>[6x]MFKDGSLIPYLTAGDPD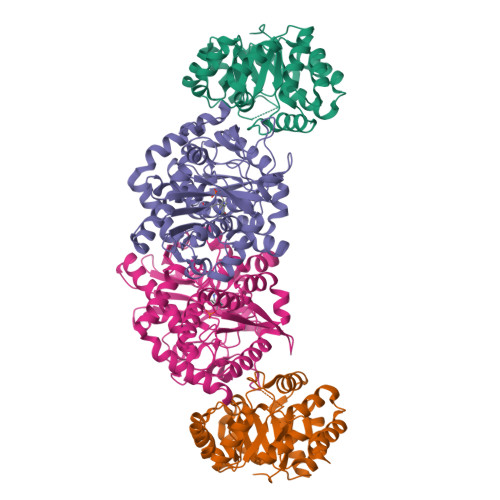KQSTLNFLLALDEYAGAIELGIPFSDPIADGKTIQESHYRALKNGFKLREAFWIVKEFRRHSSTPIVLMTYYNPIYRAGVRNFLAEAKASGVDGILVVDLPVFHAKEFTEIAREEGIKTVFLAAPNTPDERLKVIDDMTTGFVYLVSLYGTTGAREEIPKTAYDLLRRAKRICRNKVAVGFGVSKREHVVSLLKEGANGVVVGSALVKIIGEKGREATEFLKKKVEELLGI;>MWFGEFGGQYVPETLIEPLKELEKAYKRFKDDEEFNRQLNYYLKTWAGRPTPLYYAKRLTEKIGGAKIYLKREDLVHGGAHKTNNAIGQALLAKFMGKTRLIAETGAGQHGVATAMAGALLGMKVDIYMGAEDVERQKMNVFRMKLLGANVIPVNSGSRTLKDAINEALRDWVATFEYTHYLIGSVVGPHPYPTIVRDFQSVIGREAKAQILEAEGQLPDVIVACVGGGSNAMGIFYPFVNDKKVKLVGVEAGGKGLESGKHSASLNAGQVGVFHGMLSYFLQDEEGQIKPTHSIAPGLDYPGVGPEHAYLKKIQRAEYVTVTDEEALKAFHELSRTEGIIPALESAHAVAYAMKLAKEMSRDEIIIVNLSGRGDKDLDIVLKVS[6x]>[2x]GSKGVSDLLGFKIFGMPLPLYAFALITLLLSHFYNALPTDIVGGFAIMFIIGAIFGEIGKRLPIFNKYIGGAPVMIFLVAAYFVYAGIFTQKEIDAISNVMDKSNFLNLFIAVLITGAILSVNRRLLLKSLLGYIPTILMGIVGASIFGIAIGLVFGIPVDRIMMLYVLPIMGGGNGAGAVPLSEIYHSVTGRSREEYYSTAIAILTIANIFAIVFAAVLDIIGKKHTWLSGEGELVRKASFKVEEDEKTGQITHRETAVGLVLSTTCFLLAYVVAKKILPSIGGVAIHYFAWMVLIVAALNASGLCSPEIKAGAKRLSDFFSKQLLWVLMVGVGVCYTDLQEIINAITFANVVIAAIIVIGAVLGAAIGGWLMGFFPIESAITAGLCMANRGGSGDLEVLSACNRMNLISYAQISSRLGGGIVLVIASIVFGMMIPR

The 2-HCT family of transporters generally translocate molecules with a 2-hydroxycarboxylate motif (HO-CR1R2-COO−), such as citrate, malate and lactate across the plasma membrane, and activity is tightly coupled to energy provided by a sodium or proton gradient as a form of secondary active transport. Our crystal structures reveal that the KpCitS protomer is formed by homologous N-terminal and C-terminal halves with inverted topology, each containing six transmembrane helices (TM 2–5, 7 and TM 8–11, 13) and one helical hairpin (TM 6a/b (or HP1) and TM 12a/b (or HP2)). KpCitS protomer can be divided into two domains; a central dimerization domain (TM 1–4 and 8–10) critical for formation of the dimeric structure, and a peripheral transport domain (TM 5–7 and 11–13) containing residues needed for interaction with citrate and sodium ions. Our results show that the KpCitS has a homodimeric structure in which its dimerization domain remains fixed during the transport cycle due to a hydrogen bond network as well as extensive hydrophobic interactions, while the substrate-loaded transport domain undergoes an elevator-type translocation (i.e. up and down) across the membrane.

The final models showed that two crystal forms of KpCitS were obtained in the citrate-containing droplet. One crystal form (form 1), refined at 4.0 Å resolution, contains an outward-facing KpCitS homodimer. In the outward-facing state, the hairpin loops are located close to the membrane/periplasm interface, which appears to favor the entry of external substrate and ions (left). In the outward-facing state the bound citrate is partially exposed to the periplasmic space. However, it is unlikely that it can escape backwards because it is secured by strong hydrogen and electrostatic interactions. In the outward-facing conformation, L408 and I121 are in close proximity, and serve as a latch governing access of substrate to the cytoplasm. In addition, M417 seems to act as a plug preventing substrate exit.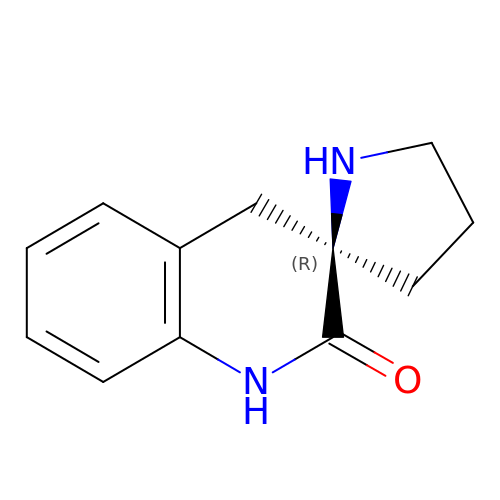(2R)-1',4'-dihydro-2'H-spiro[pyrrolidine-2,3'-quinolin]-2'-one | C12 H14 N2 O | ABOZUPQQWCLVDB-GFCCVEGCSA-N> MQTVLAKIVADKAIWVEARKQQQPLASFQNEVQPSTRHFYDALQGARTAFILECKKASPSKGVIRDDFDPARIAAIYKHYASAISVLTDEKYFQGSFNFLPIVSQIAPQPILCKDFIIDPYQIYLARYYQADACLLMLSVLDDDQYRQLAAVAHSLEMGVLTEVSNEEEQERAIALGAKVVGINNRDLRDLSIDLNRTRELAPKLGHNVTVISESGINTYAQVRELSHFANGFLIGSALMAHDDLHAAVRRVLLGENKVCGLTRGQDAKAAYDAGAIYGGLIFVATSPRCVNVEQAQEVMAAAPLQYVGVFRNHDIADVVDKAKVLSLAAVQLHGNEEQLYIDTLREALPAHVAIWKALSVGETLPAREFQHVDKYVLDNGQGGSGQRFDWSLLNGQSL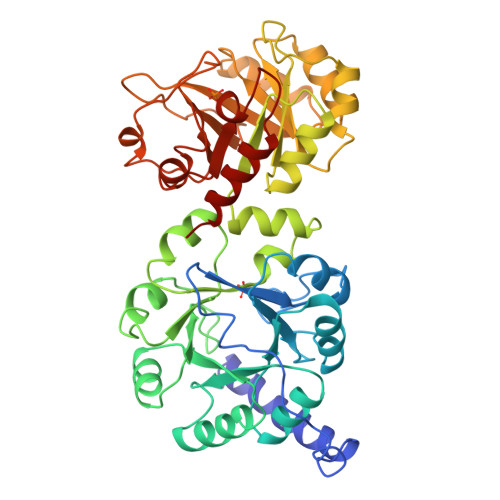GNVLLAGGLGADNCVEAAQTGCAGLDFNSAVESQPGIKDARLLASVFQTLRAY> MEILMSITVGVLFMVGTYLILTKSLLRVVVGLILLSHG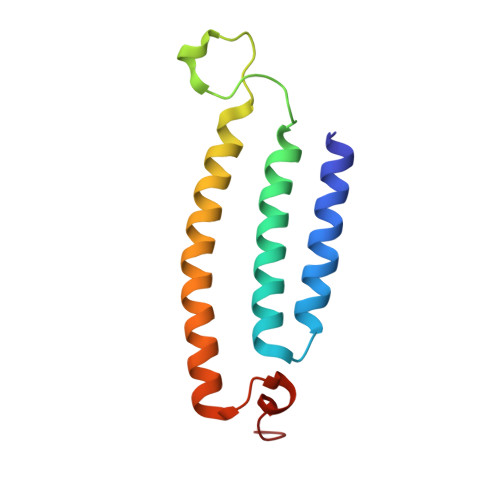AHLLLLTMAGLQRGAPPLLHLEATTYSDPLPQALILTAIVISFGVTSFLLVLAYRTYKEHKTDDLDQLRGSADE> GGAGGGGAAAUUCUAUCUGGUGAUAGACGGGAACUCUAAAUUCCUUGAAAUGCCUCGCCGCAUUGGGUUCGAUUCCCUUCCCCUCCGCCA

A search of metagenomic sequences revealed uniquely structured tRNAs (allo-tRNAs) containing recognition elements that resembled tRNASec but with a 12 bp acceptor domain (acceptor and T-stem combined) for proper recognition by EF-Tu. Specifically, tRNAUTu1 was found to be a serine isoacceptor with a 9/3 (acceptor/T-stem bp) structure that allowed EF-Tu driven Sec incorporation. Here, we investigated the suitability of an allo-tRNA, tRNAUTu1, for translation by E. coli ribosomes, and demonstrate the importance of global tRNA structure for efficient translation. tRNAUTu1 is used for site-specific insertion of Sec by harnessing EF-Tu to avoid constraints on natural Sec translation. Implementing cryo-EM, we visualized tRNAUTu1 in complex with the E. coli ribosome to pinpoint the structural feature in tRNAUTu1 hindering translation.

We made a C8A mutation to reduce the likelihood that a base pair would form with A45 (tRNAUTu1A). Data processing and particle sorting resulted with two maps, each with either A site tRNAUTu1A or P site tRNAUTu1A alone. The P site tRNAUTu1A anticodon stem, acceptor arm, and elbow region density are well defined and similar to tRNAUTu1. Highly flexible RNA chains are often poorly defined in cryo-EM, which in turn can point to higher flexibility of the variable loop of tRNAUTu1A in accordance with our single-molecule FRET data presented above. Real-time single-molecule FRET experiments confirmed that tRNAUTu1A processivity on the ribosome P site increased significantly (75%) relative to tRNAUTu1 (21%), equivalent to what was observed for tRNAsupD. Instead, the absence of the C8:A45 mismatch base pair in the core of tRNAUTu1A created flexibility in the variable arm such that it could move cooperatively with the ASF in transition from the A to the P site. This movement is likely favorable for translation and prevents ribosome disassembly.> GSNGVSEAELLTKTLP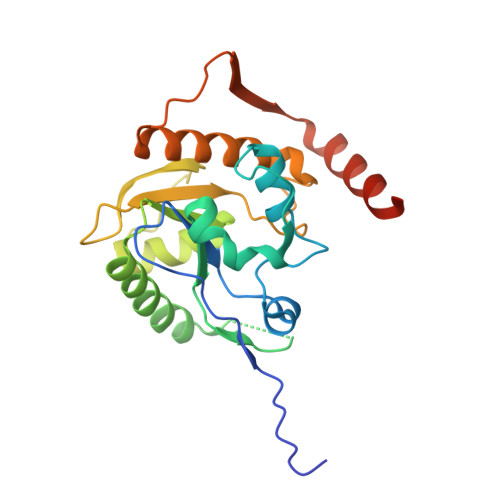DILTFNLDIVIIGINPGLMAAYKGHHYPGPGNHFWKCLFMSGLSEVQLNHMDDHTLPGKYGIGFTNMVERTTPGSKDLSSKEFREGGRILVQKLQKYQPRIAVFNGKCIYEIFSKEVFGVKVKNLEFGLQPHKIPDTETLCYVMPSSSARCAQFPRAQDKVHYYIKLKDLRDQLKGIERNMDVQEVQYTFDLQLAQEDAKKMAVKEEKYDPGYE>[8x]MSDSQTLVVKLGTSVLTGGSRRLNRAHIVELVRQCAQLHAAGHRIVIVTSGAIAAGREHLGYPELPATIASKQLLAAVGQSRLIQLWEQ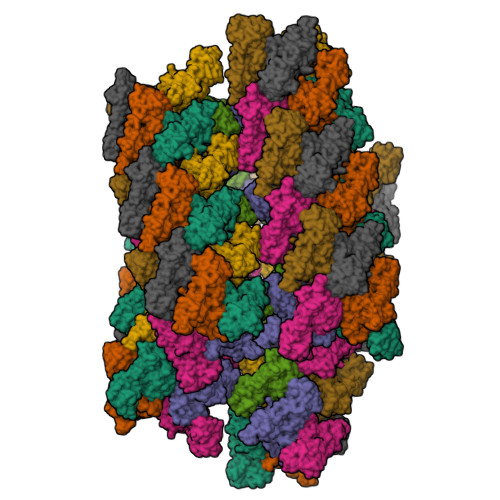LFSIYGIHVGQMLLTRADMEDRERFLNARDTLRALLDNNIVPVINENDAVATAEIKVGDNDNLSALAAILAGADKLLLLTDQKGLYTADPRSNPQAELIKDVYGIDDALRAIAGDSVSGLGTGGMSTKLQAADVACRAGIDTIIAAGSKPGVIGDVMEGISVGTLFHAQATPLENRKRWIFGAPPAGEITVDEGATAAILERGSSLLPKGIKSVTGNFSRGEVIRICNLEGRDIAHGVSRYNSDALRRIAGHHSQEIDAILGYEYGPVAVHRDDMITR(3aR,10R,10aR,11aR)-1,2,3,5,10,10a,11,11a-octahydro-3a,10-ethanopyrrolo[3',4':4,5]pyrrolo[1,2-b]isoquinolin-13-one 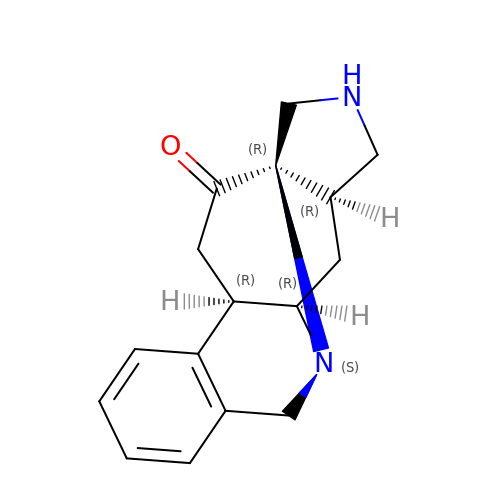| C16 H18 N2 O | JTERCRHEKKZOFH-MEWXFMAXSA-N>VPDPTSAIGVLTSGGDAQGMNAAVRAVVRMGIYVGAKVYFIYEGYQGMVDGGSNIAEADWESVSSILQVGGTIIGSARCQAFRTREGRLKAACNLLQRGITNLCVIGGDGSLTGANLFRKEWSGLLEELARNGQ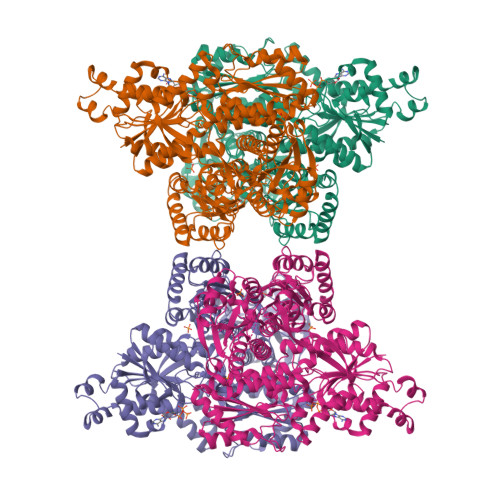IDKEAVQKYAYLNVVGMVGSIDNDFCGTDMTIGTDSALHRIIEVVDAIMTTAQSHQRTFVLEVMGRHCGYLALVSALACGADWVFLPESPPEEGWEEQMCVKLSENRARKKRLNIIIVAEGAIDTQNKPITSEKIKELVVTQLGYDTRVTILGHVQRGGTPSAFDRILASRMGVEAVIALLEATPDTPACVVSLNGNHAVRLPLMECVQMTQDVQKAMDERRFQDAVRLRGRSFAGNLNTYKRLAIKLPDDQIPKTNCNVAVINVGAPAAGMNAAVRSAVRVGIADGHRMLAIYDGFDGFAKGQIKEIGWTDVGGWTGQGGSILGTKRVLPGKYLEEIATQMRTHSINALLIIGGFEAYLGLLELSAAREKHEEFCVPMVMVPATVSNNVPGSDFSIGADTALNTITDTCDRIKQSASGTKRRVFIIETMGGYCGYLANMGGLAAGADAAYIFEEPFDIRDLQSNVEHLTEKMKTTIQRGLVLRNESCSENYTTDFIYQLYSEEGKGVFDCRKNVLGHMQQGGAPSPFDRNFGTKISARAMEWITAKLKEARGRGKKFTTDDSICVLGISKRNVIFQPVAELKKQTDFEHRIPKEQWWLKLRPLMKILA[4x]> ASELNIYSARHYNADFEIIKKFEEKTGIKVNHTQAKASELIKRLSLEGSNSPADIFITADISNLTEAKNLGLLSPVSSKYLEEFIPAHLRDKDKEWFAITKRARIIAYNKNTNIDISKMKNYEDLAKAEFKGEIVMRSATAPYSKTLLASIIANDGNKEAKAWAKGVLENLATNPKGGDRDQARQVF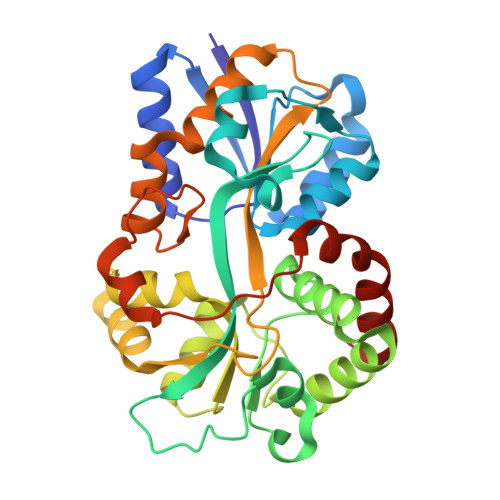AGEAKFAVMNTYYIGLLKNSKNPKDVEVGNSLGIIFPNQDNRGTHINISGIAMTKSSKNQDAAKKFMEFMLSPEIQKILTDSNYEFPIRNDVELSQTVKDFGTFKEDQIPVSKIAENIKEAVKIYDEVGFRIEGR> MPMYQVKPYHGGGAPL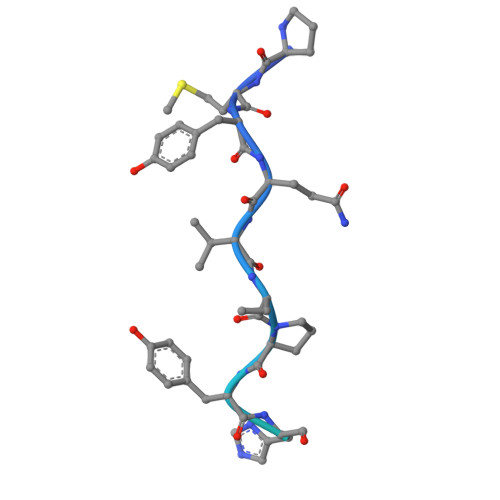RVELPTCMYRLPNVHGRSYGHHHHHH>MDTEGFGELLQQAEQLAAETEGISELPHVERNLQEIQQAGERLRSRTLTRTSQETADVKASVLLGSRGLDISHISQRLESLSAATTFEPLEPVKDTDIQGFLKNEKDNALLSAIEESRKRTFGMAEEYHRESMLVEWEQVKQRILHTLLASGEDALDFTQESEPSYISDVGPPGRSSLDNIEMAYARQIYIYNEKIVNGHLQPNLVDLCASVAELDDKSISDMWTMVKQMTDVLLTPATDALKNRSSVEVRMEFVRQALAYLEQSYKNYTLVTVFGNLHQAQLGGVPGTYQLVRSFLNIKLPAPLPGLQDGEVEGHPVWALIYYCMRCGDLLAASQVVNRAQHQLGEFKTWFQEYMNSKDRRLSPATENKLRLHYRRALRNNTDPYKRAVYCIIGRCDVTDNQSEVADKTEDYLWLKLNQVCFDDDGTSSPQDRLTLSQFQKQLLEDYGESHFTVNQQPFLYFQVLFLTAQFEAAVAFLFRMERLRCHAVHVALVLFELKLLLKSSGQSAQLLSHEPGDPPCLRRLNFVRLLMLYTRKFESTDPREALQYFYFLRDEKDSQGENMFLRCVSELVIESREFDMILGKLENDGSRKPGVIDKFTSDTKPIINKVASVAENKGLFEEAAKLYDLAKNADKVLELMNKLLSPVVPQISAPQSNKERLKNMALSIAERYRAQGISANKFVDSTFYLLLDLITFFDEYHSGHIDRAFDIIERLKLVPLNQESVEERVAAFRNFSDEIRHNLSEVLLATMNILFTQFKRLKGTSPSSSSRPQRVIEDRDSQLRSQARTLITFAGMIPYRTSGDTNARLVQMEVLMN[4x];>MATPLAVNSAASLWGPYKDIWHKVGNALWRRQPEAVHLLDKILKKHKPDFISLFKNPPKNVQQHEKVQKASTEGVAIQGQQGTRLLPEQLIKEAFILSDLFDIGELAAVELLLAGEHQQPHFPGLTRGLVAVLLYWDGKRCIANSLKALIQSRRGKTWTLELSPELASMTTRFTDELMEQGLTYKVLTLVSQIDVNNEFEKLQRERGLGSEKHRKEVSDLIKECRQSLAESLFAWACQSPLGKEDTLLLIGHLERVTVEANGSLDAVNLALLMALLYCFDISFIEQSTEERDDMIHQLPLLTEKQYIATIHSRLQDSQLWKLPGLQATVRLAWALALRGISQLPDVTALAEFTEADEAMAELAIADNVFLFLMESVVVSEYFYQEEFYIRRVHNLITDFLALMPMKVKQLRNRADEDARMIHMSMQMGNEPPISLRRDLEHLMLLIGELYKKNPFHLELALEYWCPTEPLQTPTIMGSYLGVAHQRPPQRQVVLSKFVRQMGDLLPPTIYIPYLKMLQGLANGPQCAHYCFSLLKVNGSSHVENIQGAGGSPVSWEHFFHSLMLYHEHLRKDLPSADSVQYRHLPSRGITQKEQDGLIAFLQLTSTIITWSENARLALCEHPQWTPVVVILGLLQCSIPPVLKAELLKTLAAFGKSPEIAASLWQSLEYTQILQTVRIPSQRQAIGIEVELNEIESRCEEYPLTRAFCQLISTLVESSFPSNLGAGLRPPGFDPYLQFLRDSVFLRFRTRAYRRAAEKWEVAEVVLEVFYKLLRDYEPQLEDFVDQFVELQGEEIIAYKPPGFSLMYHLLNESPMLELALSLLEEGVKQLDTYAPFPGKKHLEKAVQHCLALLNLTLQKENLFMDLLRESQLALIVCPLEQLLQGINPRTKKADNVVNIARYLYHGNTNPELAFESAKILCCISCNSNIQIKLVGDFTHDQSISQKLMAGFVECLDCEDAEEFVRLEEGSELEKKLVAIRHETRIHILNLLITSLECNPPNLALYLLGFELKKPVSTTNLQDPGVLGCPRTCLHAILNILEKGTEGRTGPVAVRESPQLAELCYQVIYQLCACSDTSGPTMRYLRTSQDFLFSQLQYLPFSNKEYEISMLNQMSWLMKTASIELRVTSLNRQRSHTQRLLHLLLDDMPVKPYSDGEGGIEDENRSVSGFLHFDTATKVRRKILNILDSIDFSQEIPEPLQLDFFDRAQIEQVIANCEHKNLRGQTVCNVKLLHRVLVAEVNALQGMAAIGQRPLLMEEISTVLQYVVGRNKLLQCLHAKRHALESWRQLVEIILTACPQDLIQAEDRQLIIRDILQDVHDKILDDEAAQELMPVVAGAVFTLTAHLSQAVLTEQKETSVLGPAEAHYAFMLDSCFTSPPPEENPLVGFASIGDSSLYIILKKLLDFILKTGGGFQRVRTHLYGSLLYYLQIAQRPDEPDTLEAAKKTMWERLTAPEDVFSKLQRENIAIIESYGAALMEVVCRDACDGHEIGRMLALALLDRIVSVDKQQQWLLYLSNSGYLKVLVDSLVEDDRTLQSLLTPQPPLLKALYTYESKMAFLTRVAKIQQGALELLRSGVIVRLAQCQVYDMRPETDPQSMFGMRDPPMFIPTPVDRYRQILLPALQLCQVILTSSMAQHLQAAGQVLQFLISHSDTIQAILRCQDVSAGSLQELALLTGIISKAALPGILSELDVDVNEGSLMELQGHIGRFQRQCLGLLSRFGGSDRLRQFKFQDDNVEGDKVSKKDEIELAMQQICANVMEYCQSLMLQSSPTFQHAVCLFTPSLSETVNRDGPRQDTQAPVVPYWRLPGLGIIIYLLKQSANDFFSYYDSHRQSVSKLQNVEQLPPDEIKELCQSVMPAGVDKISTAQKYVLARRRLVKVINNRAKLLSLCSFIIETCLFILWRHLEYYLLHCMPTDSQDSLFASRTLFKSRRLQDSFASETNLDFRSGLAIVSQHDLDQLQADAINAFGESLQKKLLDIEGLYSKVRSRYSFIQALVRRIRGLLRISRN[4x];>MPSSLLGAAMPASTSAAALQEALENAGRLIDRQLQEDRMYPDLSELLMVSAPNNPTVSGMSDMDYPLQGPGLLSVPNLPEISSIRRVPLPPELVEQFGHMQCNCMMGVFPPISRAWLTIDSDIFMWNYEDGGDLAYFDGLSETILAVGLVKPKAGIFQPHVRHLLVLATPVDIVILGLSYANLQTGSGVLNDSLSGGMQLLPDPLYSLPTDNTYLLTITSTDNGRIFLAGKDGCLYEVAYQAEAGWFSQRCRKINHSKSSLSFLVPSLLQFTFSEDDPILQIAIDNSRNILYTRSEKGVIQVYDLGQDGQGMSRVASVSQNAIVSAAGNIARTIDRSVFKPIVQIAVIENSESLDCQLLAVTHAGVRLYFSTCPFRQPLARPNTLTLVHVRLPPGFSASSTVEKPSKVHRALYSKGILLMAASENEDNDILWCVNHDTFPFQKPMMETQMTAGVDGHSWALSAIDELKVDKIITPLNKDHIPITDSPVVVQQHMLPPKKFVLLSAQGSLMFHKLRPVDQLRHLLVSNVGGDGEEIERFFKLHQEDQACATCLILACSTAACDREVSAWATRAFFRYGGEAQMRFPTTLPPPSNVGPILGSPVYSSSPVPSGSPYPNPSFLGTPSHGIQPPAMSTPVCALGNPATQATNMSCVTGPEIVYSGKHNGICIYFSRIMGNIWDASLVVERIFKSGNREITAIESSVPCQLLESVLQELKGLQEFLDRNSQFAGGPLGNPNTTAKVQQRLIGFMRPENGNPQQMQQELQRKFHEAQLSEKISLQAIQQLVRKSYQALALWKLLCEHQFTIIVAELQKELQEQLKITTFKDLVIRDKELTGALIASLINCYIRDNAAVDGISLHLQDICPLLYSTDDAICSKANELLQRSRQVQNKTEKERMLRESLKEYQKISNQVDLSNVCAQYRQVRFYEGVVELSLTAAEKKDPQGLGLHFYKHGEPEEDIVGLQAFQERLNSYKCITDTLQELVNQSKAAPQSPSVPKKPGPPVLSSDPNMLSNEEAGHHFEQMLKLSQRSKDELFSIALYNWLIQVDLADKLLQVASPFLEPHLVRMAKVDQNRVRYMDLLWRYYEKNRSFSNAARVLSRLADMHSTEISLQQRLEYIARAILSAKSSTAISSIAADGEFLHELEEKMEVARIQLQIQETLQRQYSHHSSVQDAVSQLDSELMDITKLYGEFADPFKLAECKLAIIHCAGYSDPILVQTLWQDIIEKELSDSVTLSSSDRMHALSLKIVLLGKIYAGTPRFFPLDFIVQFLEQQVCTLNWDVGFVIQTMNEIGVPLPRLLEVYDQLFKSRDPFWNRMKKPLHLLDCIHVLLIRYVENPSQVLNCERRRFTNLCLDAVCGYLVELQSMSSSVAVQAITGNFKSLQAKLERLH[4x];>MAFNFGAPSGTSGTAAATAAPAGGFGGFGTTSTTAGSAFSFSAPTNTGTTGLFGGTQNKGFGFGTGFGTTTGTSTGLGTGLGTGLGFGGFNTQQQQQTTLGGLFSQPTQAPTQSNQLINTASALSAPTLLGDERDAILAKWNQLQAFWGTGKGYFNNNIPPVEFTQENPFCRFKAVGYSCMPSNKDEDGLVVLVFNKKETEIRSQQQQLVESLHKVLGGNQTLTVNVEGTKTLPDDQTEVVIYVVERSPNGTSRRVPATTLYAHFEQANIKTQLQQLGVTLSMTRTELSPAQIKQLLQNPPAGVDPIIWEQAKVDNPDSEKLIPVPMVGFKELLRRLKVQDQMTKQHQTRLDIISEDISELQKNQTTSVAKIAQYKRKLMDLSHRTLQVLIKQEIQRKSGYAIQADEEQLRVQLDTIQGELNAPTQFKGRLNELMSQIRMQNHFGAVRSEERYYIDADLLREIKQHLKQQQEGLSHLISIIKDDLEDIKLVEHGLNETIHIRGGVFS[4x];>MSTGFSFGSGTLGSTTVAAGGTSTGGVFSFGTGASSNPSVGLNFGNLGSTSTPATTSAPSSGFGTGLFGSKPATGFTLGGTNTGIATTITTGLTLGTPATTSAATTGFSLGFNKPAASATPFALPITSTSASGLTLSSALTSTPAASTGFTLNNLGGTTATTTTASTGLSLGGALAGLGGSLFQSTNTGTSGLGQNALGLTLGTTAATSTAGNEGLGGIDFSSSSDKKSDKTGTRPEDSKALKDENLPPVICQDVENLQKFVKEQKQVQEEISRMSSKAMLKVQEDIKALKQLLSLAANGIQRNTLNIDKLKIETAQELKNAEIALRTQKTPPGLQHEYAAPADYFRILVQQFEVQLQQYRQQIEELENHLATQANNSHITPQDLSMAMQKIYQTFVALAAQLQSIHENVKVLKEQYLGYRKMFLGDAVDVFETRRAEAKKWQNTPRVTTGPTPFSTMPNAAAVAMAATLTQQQQPATGPQPSLGVSFGTPFGSGIGTGLQSSGLGSSNLGGFGTSSGFGCSTTGASTFGFGTTNKPSGSLSAGFGSSSTSGFNFSNPGITASAGLTFGVSNPASAGFGTGGQLLQLKKPPAGNKRGKR[4x];>MSGFNFGGTGAPTGGFTFGTAKTATTTPATGFSFSTSGTGGFNFGAPFQPATSTPSTGLFSLATQTPATQTTGFTFGTATLASGGTGFSLGIGASKLNLSNTAATPAMANPSGFGLGSSNLTNAISSTVTSSQGTAPTGFVFGPSTTSVAPATTSGGFSFTGGSTAQPSGFNIGSAGNSAQPTAPATLPFTPATPAATTAGATQPAAPTPTATITSTGPSLFASIATAPTSSATTGLSLCTPVTTAGAPTAGTQGFSLKAPGAASGTSTTTSTAATATATTTSSSSTTGFALNLKPLAPAGIPSNTAAAVTAPPGPGAAAGAAASSAMTYAQLESLINKWSLELEDQERHFLQQATQVNAWDRT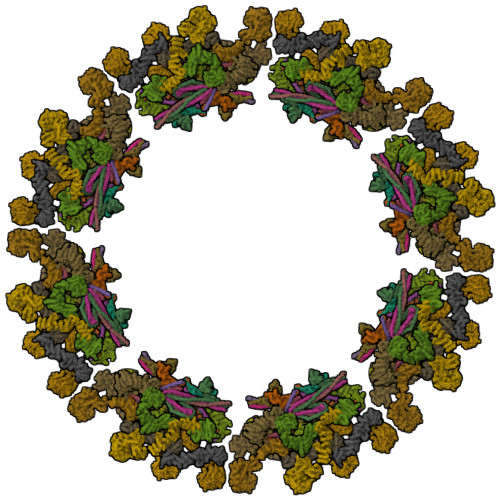LIENGEKITSLHREVEKVKLDQKRLDQELDFILSQQKELEDLLSPLEELVKEQSGTIYLQHADEEREKTYKLAENIDAQLKRMAQDLKDIIEHLNTSGAPADTSDPLQQICKILNAHMDSLQWIDQNSALLQRKVEEVTKVCEGRRKEQERSFRITFD[4x]(2R)-1-[(4-tert-butylphenyl)sulfonyl]-2-methyl-4-(4-nitrophenyl)piperazine | C21 H27 N3 O4 S | 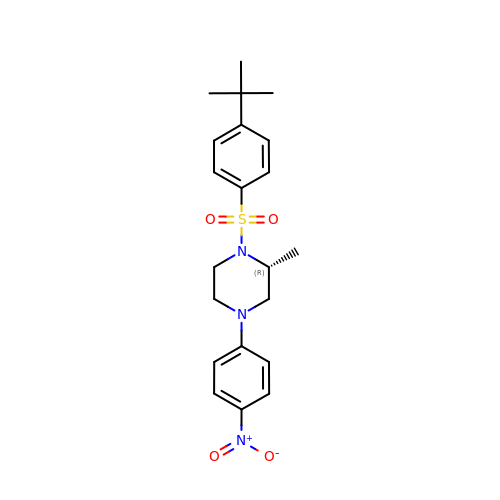SOFGQQQVQZQJFS-MRXNPFEDSA-N> NSVTYNTLISGLGKAGRLEEALELFEEMKEKGIVPDVVTYNTLISGLGKAGRLEEALELFEEMKEKGIVPDVVTYTTLISGLGKAGRLEEALELFEEMKEKGIVPNVVTYTTLISGLGKAGRLEEALELFEEMKEKGIVPDVVTYTTLISGLGKAGRLEEALELFEEMKEKGIVPDVVTYTTLISGLGKAGRLEEALELFEEMKEKGIVPDVVTYNTLISGLGKAGRLEEALELFEEMKEKGIVPDVVTYNTLISGLGKAGRLEEALELFEEMKEKGIVPDVVTYTTLISGLGKAGRLEEALELFEEMKEKGIVPNVVTYTTLISGLGKAGRLEEALELFEEMKEKGIVPDVVTYTTLISGLGK

PPR proteins are RNA-binding proteins found predominantly in mitochondria and chloroplasts. PPRs stack on each other to form an extended solenoid structure that can recognise RNA in a sequence-specific manner based on the identities of amino acids at positions 5 and 35 of each repeat. To bypass these limitations, we previously used consensus design to engineer artificial PPR domains (cPPRs) that are highly soluble and, via an appropriate choice of amino acids at position 5 and 35, can be designed to bind RNA in a predictable, sequence-specific manner. In this study we have discovered that cPPRs bind not only RNA but also ssDNA in a modular and programmable manner, analogous to their RNA-binding capability.

Although these proteins are highly similar in their primary sequences, only cPPR-Telo1 gave reproducible and diffracting crystals. We solved the structure of cPPR-Telo1 and cPPR-Telo1 bound to its ssDNA target using single-wavelength anomalous dispersion at 2.1 and 2.0 Å resolution, respectively (with sample electron densities in Supplementary Fig. 8). Our structures provide the first pair of structures where an identical PPR protein compacts upon binding a nucleic acid in the canonical, sequence-specific mode, providing an opportunity to understand how the conformation of the protein changes upon ligand binding. cPPR-Telo1 wraps around the ssDNA upon binding, inducing a massive compaction of the superhelical structure and decreasing the length of the protein from 104 to 64 Å. This conformational change more than halves the number of cPPR protein side chains exposed to water and may be the principal driving force favouring nucleic acid binding. To allow the separation, an extensive hydrogen bond network between an arginine at position 16 and a glutamic acid at position 19 from one PPR repeat and a glutamic acid at position 18 from the preceding repeat in the apo protein rearranges at three out of nine possible positions leading to a more open arrangement when bound to DNA. Specifically, the side chains of Glu128, Glu198 and Glu303 form hydrogen bonds to their own main chain instead of to Arg125, Arg195 and Arg300, respectively. We observed the same binding mode in our cPPR-ssDNA structure and likewise the bases were sandwiched between the valine residues at position 2 of each repeat. An identical mode of thymine recognition is seen in our structure when ssDNA is bound and the methyl group at position C5 that distinguishes uracil and thymine is orientated away from the protein, such that it is initially hard to predict why poly(T) ssDNA is bound much less efficiently than poly(U) RNA, based on this difference. Support for this hypothesis comes from the observation that although the electron density is very clear for all nucleotides, it is weaker for one of the thymines (T7) in the structure. One interesting exception is the thymine at position 1, which does not make any specific hydrogen bonds with the protein in our structure.>[4x]GDKPIAEQIGSSFIQHYYQLFDNDRTQLGAIYIDASCLTWEGQQFQGKAAIVEKLSSLPFQKIQHSITAQDHQPTPDSCIISMVVGQLKADEDPIMGFHQ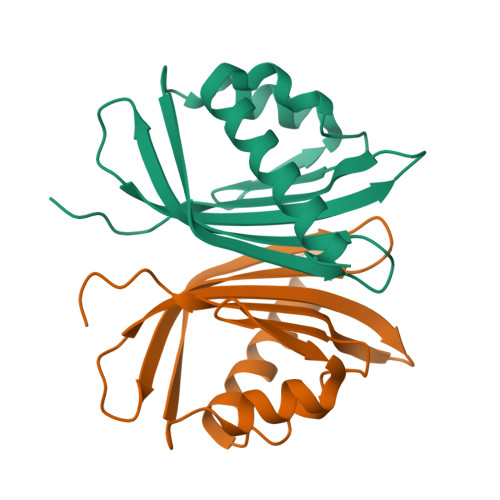MFLLKNINDAWVCTNDMFRLALHNFG>[6x]MAPKSSSSGSKKKSSASSNSADAKASKFKLPAEFITRPHPSKDHGKETCTAYIHPNVLSSLEINPGSFCTVGKIGENGILVIARAGDEEVHPVNVITLSTTIRSVGNLILGDRLELKKAQVQPPYATKVTVGSLQGYNILECMEEKVIQKLLDDSGVIMPGMIFQNLKTKAGDESIDVVITDASDDSLPDVSQLDLNMDDMYGGLDNLFYLSPPFIFRKGSTHITFSKETQANRKYNLPEPLSYAAVGGLDKEIESLKSAIEIPLHQPTLFSSFGVSPPRGILLHGPPGTGKTMLLRVVANTSNAHVLTINGP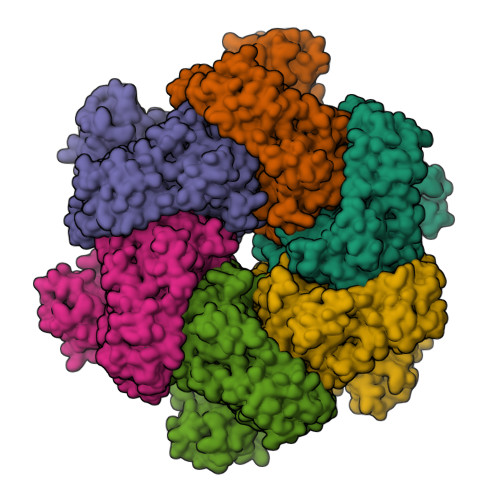SIVSKYLGETEAALRDIFNEARKYQPSIIFIDEIDSIAPNRANDDSGEVESRVVATLLTLMDGMGAAGKVVVIAATNRPNSVDPALRRPGRFDQEVEIGIPDVDARFDILTKQFSRMSSDRHVLDSEAIKYIASKTHGYVGADLTALCRESVMKTIQRGLGTDANIDKFSLKVTLKDVESAMVDIRPSAMREIFLEMPKVYWSDIGGQEELKTKMKEMIQLPLEASETFARLGISAPKGVLLYGPPGCSKTLTAKALATESGINFLAVKGPEIFNKYVGESERAIREIFRKARSAAPSIIFFDEIDALSPDRDGSSTSAANHVLTSLLNEIDGVEELKGVVIVAATNRPDEIDAALLRPGRLDRHIYVGPPDVNARLEILKKCTKKFNTEESGVDLHELADRTEGYSGAEVVLLCQEAGLAAIMEDLDVAKVELRHFEKAFKGIARGITPEMLSYYEEFALRSGSSS> MTADELVFFVNGKKVVEKNADPETTLLAYLRRKLGLRGTKLGCGEGGCGACTVMLSKYDRLQDKIIHFSANACLAPICTLHHVAVTTVEGI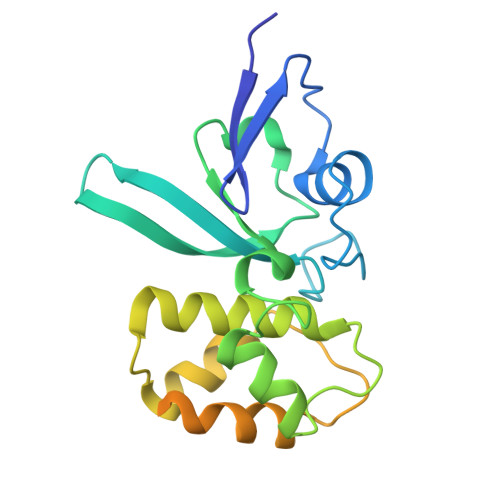GSTKTRLHPVQERIAKSHGSQCGFCTPGIVMSMYTLLRNQPEPTVEEIEDAFQGNLCRCTGYRPILQGFRTFAKNGGCCGGNGNNPNCCMNQKKDHTVTLSPSLFNPEEFMPLDPTQEPIFPPELLRL> MQDAITAVINSADVQGKYLDGAAMDKLKSYFASGELRVRAASVISANAATIVKEAVAKSLLYSDVTRPGGNMYTTRRYAACIRDLDYYLRYATYAMLAGDASILDERVLNGLKETYNSLGVPISS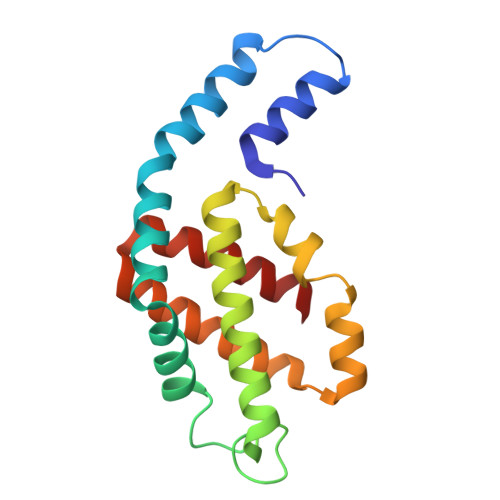TVQAIQAIKEVTASLVGADAGKEMGVYLDYICSGLS> MKRRFTLLGSVVALALSSTALASDAPASRGCADDAGWNDPAMPLKVYGNTWYVGTCGISALLVTSDAGHILVDAATPQAGPQILANIRALGFRPEDVRAIVFSHEHFDHAGSLAELQKATGAPVYARAPAIDTLKRGLPDRTDPQFEVAEPVAPVANIVTLADDGVVSVGPLALTAVASPGHTPGGTSWTWRSCEGDDCRQMVYADSLTAISDDVFRYSDDAAHPGYLAAFRNTLARVAALDCD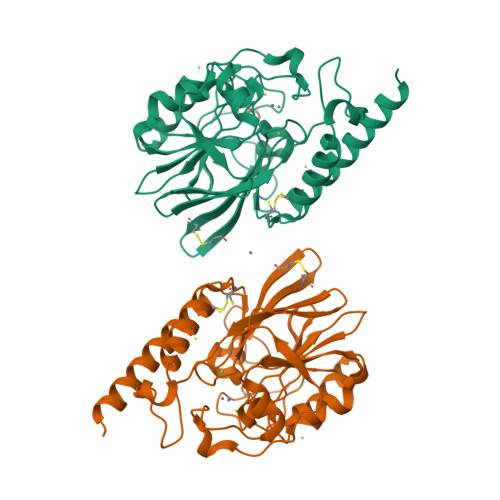ILVTPHPSASGLWNRIGPRAAAPLMDTTACRRYAQGARQRLEKRLAEEAATSPSSGARP> AMSDLELRQCLPCGPGGKGRCFGPSICCGDELGCFVGTAEALRCQEENYLPSPCQSGQKPCGSGGRCAAAGICCNDESCVTEPECREGVGFPRRV;>CYIQNCPLG[2x];> AMSDLELRQCLPCGPGGAGRCFGPSICCGDELGCFVGTAEALRCQEENYLPSPCQSGQ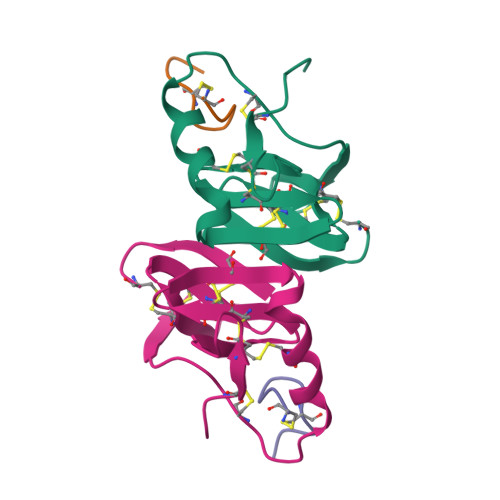KPCGSGGRCAAAGICCNDESCVTEPECREGVGFPRRV> CQPIFLNVLEAIEPGVVCAGHDNNQPDSFAALLSSLNELGERQLVHVVKWAKALPGFRNLHVDDQMAVIQYSWMGLMVFAMGWRSFTNVNSRMLYFAPDLVFNEYRMHKSRMYSQCVRMRHLSQEFGWLQITPQEFLCMKALLLFSIIPVDGLKNQKFFDELRMNYIKELDRIIACKRKNPTSCSRRFYQ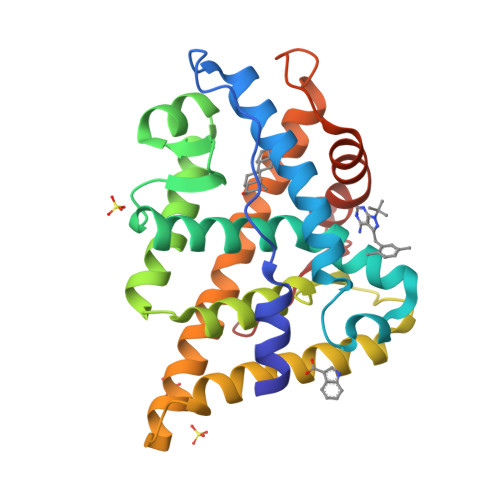LTKLLDSVQPIARELHQFTFDLLIKSHMVSVDFPEMMAEIISVQVPKILSGKVKPIYFHTQ(4S)-4-(2-fluorophenyl)-2,4,6,7,8,9-hexahydro-5H-pyrazolo[3,4-b][1,7]naphthyridin-5-one 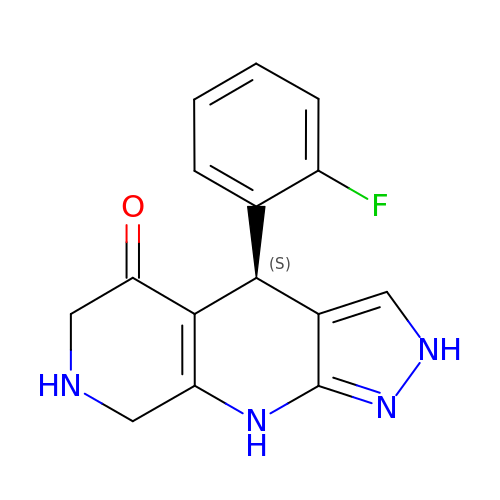| C15 H13 F N4 O | ITULOGMVDYUWCK-ZDUSSCGKSA-N> APTAVEKRASCTFTDAASAMASKTACSTITLNNIAVPAGTTLDLTGLTSGTRVIFEGTTTFGYQEWS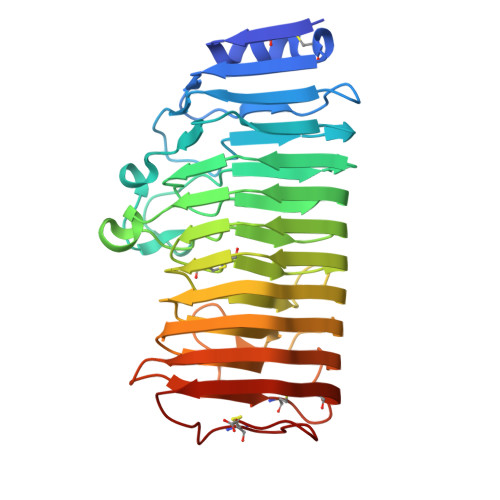GPLVSISGTDITVQGASGSVLDGDGARWWDGQGSNGGKTKPKFFYAHSLDSSSITGITIKNSPVQVFSIQSNNLSLTDITVDDADGDTQGGHNTDAFDIGSSTYITITNANVHNQDDCIAVNSGENIIFTGGTCTGGHGLSIGSVGGRSDNTVKNVTIEHSTVTNSQNGVRIKTVYGATGSVSEVTYSNIQMSGITNYGIVIEQDYENGSPTGTPTNGVPITDLTLNTVTGSVSSGATEIYILCGSGSCSSWTWTGVSITGGSKSTKCENVPSGVSC>MFSAGHKIKGTVVLMPKNELEVNPDGSAVDNLNAFLGRSVSLQLISATKADAHGKGKVGKDTFLEGINTSLPTLGAGESAFNIHFEWDGSMGIPGAFYIKNYMQVEFFLKSLTLEAISNQGTIRFVCNSWVYNTKLYKSVRIFFANHTYVPSETPAPLVEYREEELKSLRGNGTGERKEYDRIYDYDVYNDLGNPDKSEKLARPVLGGSSTFPYPRRGRTGRGPTVTDPNTEKQGEVFYVPRDENLGHLKSKDALEIGTKSLSQIVQPAFESAFDLKSTPIEFHSFQDVHDLYEGGIKLPRDVISTIIPLPVIKELYRTDGQHILKFPQPHVVQVSQSAWMTDEEFAREMIAGVNPCVIRGLEEFPPKSNLDPAIYGDQSSKITADSLDLDGYTMDEALGSRRLFMLDYHDIFMPYVRQINQLNSAKTYATRTILFLREDGTLKPVAIELSLPHSAGDLSAAVSQVVLPAKEGVESTIWLLAKAYVIVNDSCYHQLMSHWLNTHAAMEPFVIATHRHLSVLHPIYKLLTPHYRNNMNINALARQSLINANGIIETTFLPSKYSVEMSSAVYKNWVFTDQALPADLIKRGVAIKDPSTPHGVRLLIEDYPYAADGLEIWAAIKTWVQEYVPLYYARDDDVKNDSELQHWWKEAVEKGHGDLKDKPWWPKLQTLEDLVEVCLIIIWIASALHAAVNFGQYPYGGLIMNRPTASRRL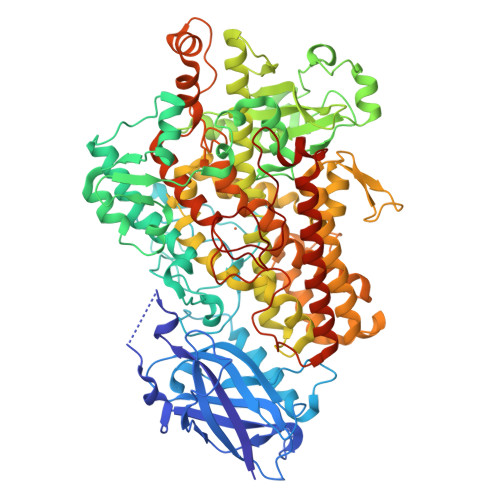LPEKGTPEYEEMINNHEKAYLRTITSKLPTLISLSVIEILSTHASDEVYLGQRDNPHWTSDSKALQAFQKFGNKLKEIEEKLVRRNNDPSLQGNRLGPVQLPYTLLYPSSEEGLTFRGIPNSISI[2x]> MSHPDYRMNLRPLGTPRGVSAVAGPHDIGASPGDKKSKNRSTRGKKKSIFETYMSKEDVSEGLKRGTLIQGVLRINPKKFHEAFIPSPDGDRDIFIDGVVAR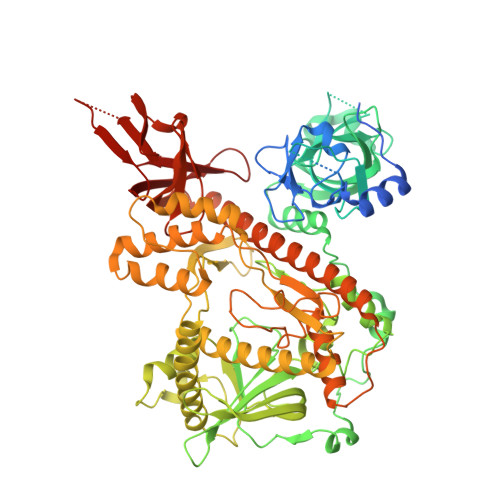NRALNGDLVVVKLLPEEHWKVVKPESNDKETEAAYESDIPEELCGHHLPQQSLKSYNDSPDVIVEAQFDGSDSEDGHGITQNVLVDGVKKLSVCVSEKGREDGDAPVTKDETTCISQDTRALSEKSLQRSAKVVYILEKKHSRAATGFLKLLADKNSELFRKYALFSPSDHRVPRIYVPLKDCPQDFVARPKDYANTLFICRIVDWKEDCNFALGQLAKSLGQAGEIEPETEGILTEYGVDFSDFSSEVLECLPQGLPWTIPPEEFSKRRDLRKDCIFTIDPSTARDLNDALSCKPLADGNFKVGVHIADVSYFVPEGSDLDKVAAERATSVYLVQKVVPMLPRLLCEELCSLNPMSDKLTFSVIWTLTPEGKILDEWFGRTIIRSCTKLSYEHAQSMIESPTEKIPAKELPPISPEHSSEEVHQAVLNLHGIAKQLRQQRFVDGALRLDQLKLAFTLDHETGLPQGCHIYEYRESNKLVEEFMLLANMAVAHKIHRAFPEQALLRRHPPPQTRMLSDLVEFCDQMGLPVDFSSAGALNKSLTQTFGDDKYSLARKEVLTNMCSRPMQMALYFCSGLLQDPAQFRHYALNVPLYTHFTSPIRRFADVLVHRLLAAALGYRERLDMAPDTLQKQADHCNDRRMASKRVQELSTSLFFAVLVKESGPLESEAMVMGILKQAFDVLVLRYGVQKRIYCNALALRSHHFQKVGKKPELTLVWEPEDMEQEPAQQVITIFSLVEVVLQAESTALKYSAILK>MAHHHHHHMTALLREVIGDVLRNARTDQGRTLREVSDAARVSLGYLSEVERGRKEASSELLSAICDALDVPLSRVLTDAGESMARREH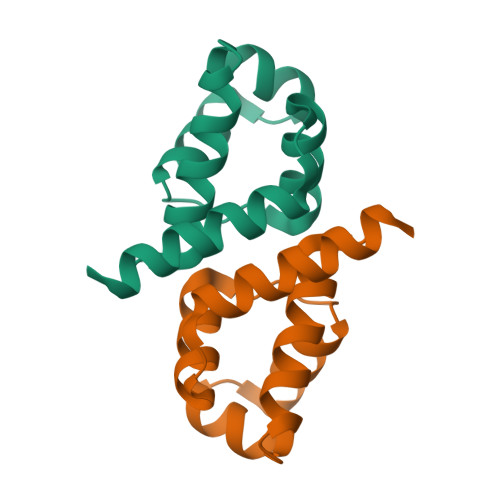DAREAEQVAVANLGRIDAATKVVIPQVSMAVA[3x]>[4x]ANSKEVKKRASSFEWF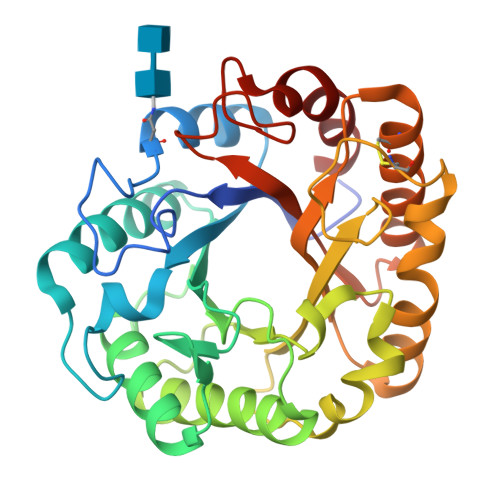GSNESGAEFGSGNIPGVEGTDYTFPNTTAIQILIDAGMNIFRVPFLMERMIPTEMTGSLDTAYFEGYSEVINYITGKGAHAVVDPHNFGRYYGTPISSTSDFQTFWSTLASQFKSNDLVIFDTNNEYHDMDESVVVALNQAAIDGIRDAGATTQYIFVEGNAYSGAWTWTTYNTAMVNLTDPSDLIVYEMHQYLDSDGSGTSDQCVSSTVGQERVVDATTWLQSNGKLGILGEFAGGANSVCEEAVEGMLDYLAENSDVWLGASWWSAGPWWQDYIYSMEPPNGIAYESYLPILETYF>KKHTGYVGLKNQGATCYMNSLLQTLFFTNQLRKAVYMMPTEGDDSSKSVPLALQRVFYELQHSDKPVGTKKLTKSFGWETLDSFMQHDVQELCRVLLDNVENKMKGTCVEGTIPKLFRGKMVSYIQCKEVDYRSDRREDYYDIQLSIKGKKNIFESFVDYVAVEQLDGDNKYDAGEHGLQEAEKGVKFLTLPPVLHLQLMRFMYDPQTDQNIKINDRFEFPEQLPLDEFLQKTDPKDPANYILHAVLVHSGDNHGGHYVVYLNPKGD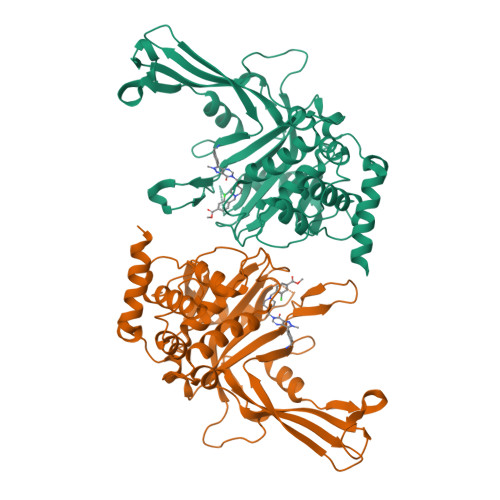GKWCKFDDDVVSRCTKEEAIEHNYGGHDDDLSVRHCTNAYMLVYIRESKLSEVLQAVTDHDIPQQLVERLQEEKRIEAQK[2x]>[3x]MKHHHHHHMSLDAFEILTTSGVVLWSRTYAPVNPSVVNDFITDVFIEEKSAVAGSKNGGSAASNPPYKHDQHSLRWTFVKELGIIFVAVY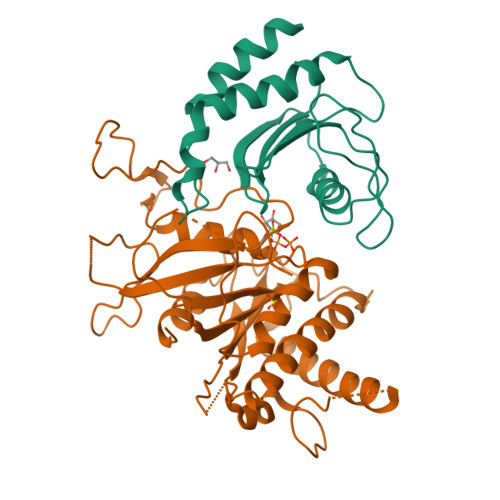RSLLHLPWVDKLVDNIRAIFVSLYSEQFKRPNTTIIECINFDKYFDQQLQELEQTGSRVDARVPKIEAHSADEEEQPFVPSPAGKSEQKAP;>[3x]MGATTQYTTLPSVLLIGPSGAGKTALLTLFERGPLLNPDGTSVGAADLKNPYRKPIVTSPVAQTHTSQVPTSVELAVGANEDGTPTSYKVDLDAAGATARKFLLIDTPGHPKLRGTTLQHLLNPSPSLTIIPTNAPNKKTSTDSHSDPYKSKLKAVIFLLDAAALADSDGDYLSQTASYLYDVLLSLQKRFHSRKNSRAPSSIPVLIAANKQDLFTAVPASLVKSRLEHELGRIRKTRQKGLLEASVTSEDEIRADDEEGWLGAVGSKEFKFEEMMEFDMEVEVMGGNVIGDGPGAERWWRWIGERI> MRGSHHHHHHGSMRHQMSWNGKDERKLSVQERGFSLEVDGRTVPGVYWSPAEGSSDRLVLLGHGGTTHKKVEYIEQVAKLLVGRGISAMAIDGPGHGERASVQAGREPTDVVGLDAFPRMWHEGGGTAAVIADWAAALDFIEAEEGPRPTGWWGLSMGTMMGLPVTASDKRIKV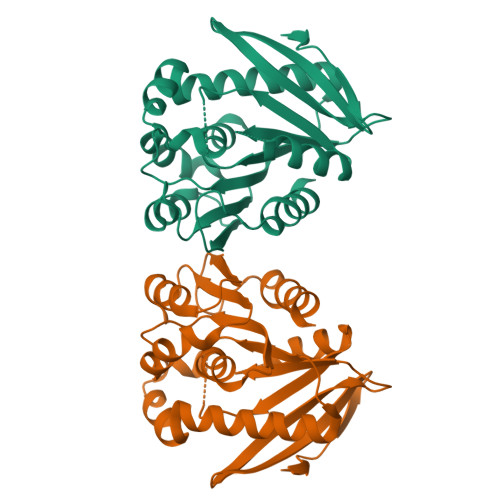ALLGLMGVEGVNGEDLVRLAPQVTCPVRYLLQWDDELVSLQSGLELFGKLGTKQKTLHVNPGKHSAVPTWEMFAGTVDYLDQRLK> QEFTIDFSTQQSYVSSLNSIRTAISTPLEHISQGATSVSVINHTPPGSYISVGIRGLDVYQAHFDHLRLIIEQNNLYVAGFVNTATNTFYRFSDFAHISLPGVTTISMTTDSSYTTLQRVAALERSGMQISRHSLVSSYLALMEFSGNTMTREASRAVLRFVTVTAQALRFRQIQREFRQALSETAPVYTMTPEDVDLTLNWGRIS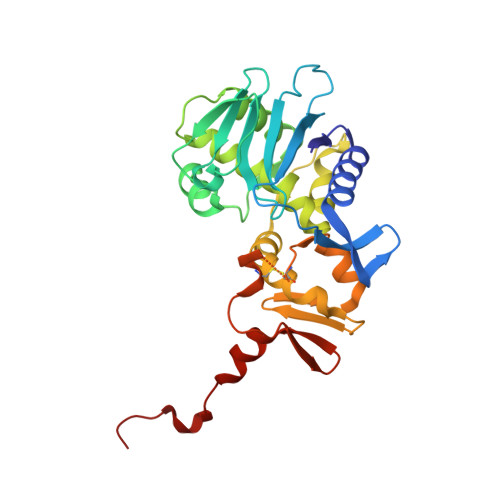NVLPEYRGEDGVRVGRISFNNISAILGTVAVILNCHHQGARSVRAVNEESQPECQITGDRPVIKINNTLWESNTAAAFLNRKSQSLYTTGE>MHCDLPCGVYDPAQARIEAESVKAVQEKMAGNDDPHFQTRATVIKEQRAELAKHHVSVLWSDYFKPPHFEKYPELH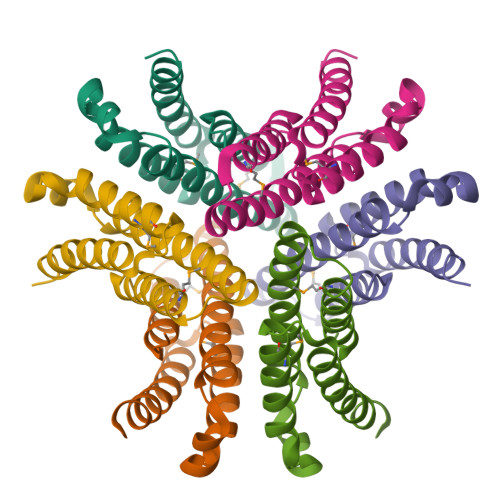QLVNDTLKAMSAAKGSKDPATGQKALDYIAQIDKIFWETKKA[3x]>GUGUACAC[6x]

To investigate and compare the uracil roles played in these non-canonical and canonical pairs, we have decided to probe the U•U and U-A pairs with a Se atom, where the exo-4-oxygen of uracil is replaced by selenium. Herein, we report the first synthesis of the 4-Se-uridine phosphoramidite (SeU) and the corresponding SeU-RNAs by replacing 4-oxygen with selenium. The rationales of using a Se atom to probe the U-A and U•U base pairs are that selenium, a large-size atom, can probably strengthen the stacking interaction and is a poorer hydrogen-bond acceptor that can likely weaken the hydrogen-bond (H-bond) interaction. To investigate the Se-nucleobase modification and its structural property, we have crystallized two Se-RNA sequences [hexamer (5′-rU-SeU-CGCG-3′)2 with overhangs and octamer (5′-rGUG-SeU-ACAC-3′)2 with a perfect duplex].

The Se-octamer structure, where the two Se atoms point to the major groove, reveals formation of the SeU-A pair and the typical right-handed A-form duplex by the Se-RNA. Moreover, we have superimposed the structures of SeU-A (or SeU4-A13 pair) and U2-A15 pair, as the corresponding native structure is not available (from literature or us) for direct comparison. This comparison of the base pair structures has demonstrated that the Se-modified and native U-A pairs are similar. The major difference is the slight shift of the SeU nucleobase to accommodate the large selenium atom, revealing the flexibility of RNA duplex structure. The distance between SeU4 exo-Se4 and A13 exo-N6 is 3.54 Å, which was increased from the original 2.99 Å. Considering that the atomic size of Se is 0.43 Å larger than that of O and that a typical H-bond length is 2.8–3.2 Å, this distance (3.54 Å) suggests a weak hydrogen bond after the Se-modification. On the other hand, the polarizable and large Se atom with delocalizable electrons may facilitate the base stacking interaction, supported by the narrower base-pair gap and the computational study of the Se-nucleobase-modified DNA. Using the Se atom probe, we found that the increased stacking interaction can compensate the loss of the H-bond interaction, which is consistent with the virtually identical duplex stability after the Se-modification. In the crystal lattice, the duplexes are stacked on the top of each other in a head-to-tail fashion and three Se-RNA duplexes present in an asymmetric unit, where the three duplexes are virtually identical (r.m.s < 0.1 Å).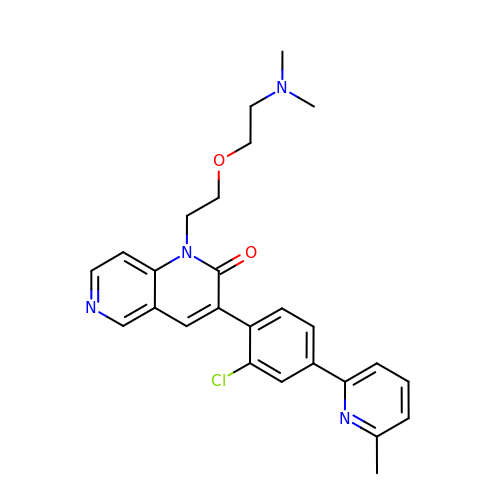(3M)-3-[(4P)-2-chloro-4-(6-methylpyridin-2-yl)phenyl]-1-{2-[2-(dimethylamino)ethoxy]ethyl}-1,6-naphthyridin-2(1H)-one | C26 H27 Cl N4 O2 | NPOXYSJSLYNRSE-UHFFFAOYSA-N> R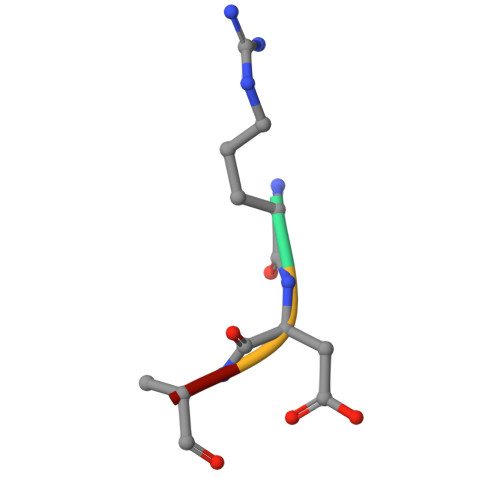DAA> MSAS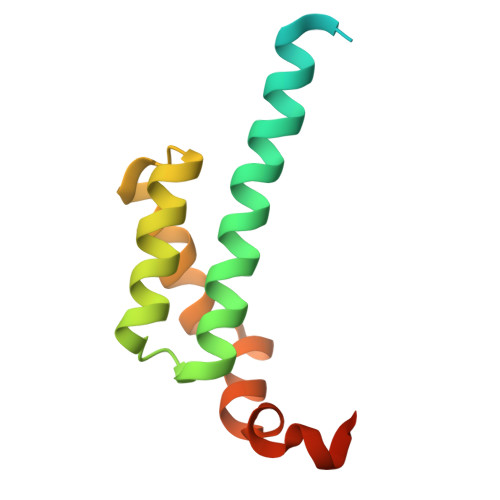GSGVAAIYGRAEEAQNAPVKLQPVPAFELYKAAREEELCSYRSLCRVLCMHSGGKLTKQQRRILEDMREELCLPTERAEAELAAAREDVLVTSVAASGVLKRRQDLEHHHHHH>MHHHHHHSN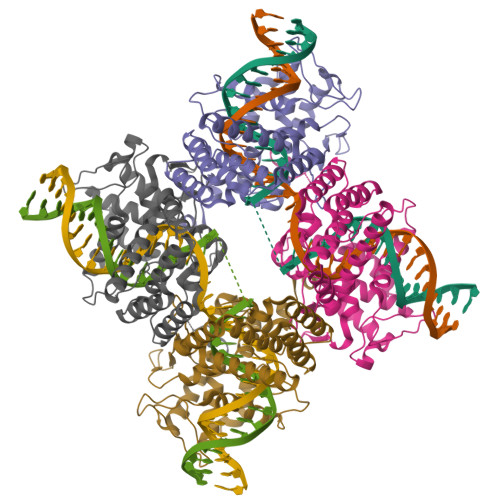LLTVHQNLPALPVDATSDEVRKNLMDMFRDRQAFSEHTWKMLLSVCRSWAAWCKLNNRKWFPAEPEDVRDYLLYLQARGLAVKTIQQHLGQLNMLHRRSGLPRPSDSNAVSLVMRRIRKENVDAGERAKQALAFERTDFDQVRSLMENSDRCQDIRNLAFLGIAYNTLLRIAEIARIRVKDISRTDGGRMLIHIGRTKTLVSTAGVEKALSLGVTKLVERWISVSGVADDPNNYLFCRVRKNGVAAPSATSQLSTRALEGIFEATHRLIYGAKDDSGQRYLAWSGHSARVGAARDMARAGVSIPEIMQAGGWTNVNIVMNYIRNLDSETGAMVRLLEDGD[2x]>MAHHHHHHVGTFENITAAPADPILGLADLFRADERPGKINLGIGVYFDETGKCPVLTSVKKAEQYLLENETTKSYLGIDGIPEFGRCTQELLFGKGSALINDKRARTAQTPGGTGALRVAADFLAKNTSVKRVWVSNPSWPNHKSVFNSAGLEVREYAYYDAENHTLDFDALINSLNEAQAGDVVLFHGCCHNPTGIDPTLEQWQTLAQLSVEKGWLPLFDFAYQGFARGLEEDAEGLRAFAAMHKELIVASSYSKNFGLYNERVGACTLVAADSETVDRAFSQMKAAIRANYSNPPAHGASVVATILSNDALRAIWEQELTDMRQRIQRMRQLFVNTLQEKGANRDFSFIIKQNGMFSFSGLTKEQVLRLREEFGVYAVASGRVNVAGMTPDNMAPLCEAIVAVL[2x]

E. coli aspartate aminotransferase (AAT) is a pyridoxal phosphate (PLP)-dependent enzyme that catalyses the reversible transamination of l-aspartate with α-ketoglutarate, yielding oxaloacetate and l-glutamate. During its catalytic cycle, AAT undergoes hinge movement to switch between an open conformation, in the ligand-free form, and a closed conformation upon association with substrates or inhibitors. Using our approach, we enrich the less populated but catalytically active closed conformation in order to increase catalytic efficiency (kcat/KM) with the non-native substrate l-phenylalanine, leading to altered substrate selectivity. Steady-state kinetics reveal kcat/KM increases of up to 100-fold towards this aromatic amino acid, resulting in a selectivity switch of up to 1900-fold, and structural analyses by room-temperature X-ray crystallography and multitemperature nuclear magnetic resonance (NMR) spectroscopy confirm that the conformational landscape is remodeled to favor the target state.

We crystallized WT, HEX, and select variants from the Closed (VFIT and VFIY), OpenLow (VFCS), and OpenHigh (AIFS) libraries. To obtain structures in the absence of maleate, we applied a rigorous crystal soaking method to serially dilute and extract the inhibitor from the crystallized enzymes. Superposition of bound and unbound structures for each variant confirmed that closed library mutants VFIT and VFIY remained in the closed conformation in the inhibitor-free form, similar to HEX, while OpenLow variant VFCS and OpenHigh variant AIFS adopted the open conformation, similar to WT. Overlay of AAT structures (Chain A) in the presence and absence of maleate show transition from open to closed states upon inhibitor binding for WT, VFCS, and AIFS, but not for HEX, VFIT, and VFIY, which already adopt the closed conformation in the absence of bound inhibitor. Interestingly, the amplitude of the open/closed conformational transition that occurs in open variants upon maleate binding correlated with their computed ΔE values (VFCS < WT < AIFS), suggesting that this metric can be used to fine-tune this enzyme conformational landscape. Furthermore, DynDom analyses of all variants confirmed that only WT, VFCS, and AIFS undergo hinge motion upon maleate binding, which rotates the moving domain relative to the fixed domain by 4.6, 2.6, and 5.9 degrees, respectively. OpenLow mutant VFCS showed 19F NMR spectra that were very similar to those of WT within the tested temperature range, consistent with its preference for the open conformation. OpenLow mutants had lower KM values and were more catalytically efficient than WT with both l-phenylalanine and l-aspartate, which could be due to the fact that these mutants have ΔE values similar to the WT but stabilize both the open and closed conformations by >10 kcal mol‒1.>[2x]GSWEIDPKDLTFLKELGTGQFGVVKYGKWRGQYDVAIKMIKEGSMSEDEFIEEAKVMMNLSHEKLVQLYGVCTKQRPIFIITEYMANGCLLNYLREMRHRFQTQQLLEMCKDVCEAMEYLESKQFLHRDLAARNCLVNDQGVVKVSDFGLSRYVLDDEYTSSVGSKFPVRWSPPEVLMYSKFS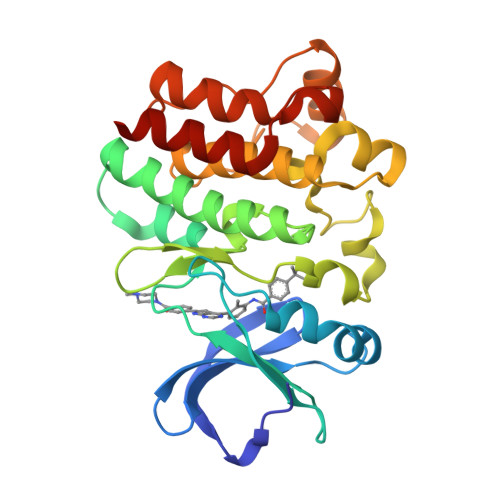SKSDIWAFGVLMWEIYSLGKMPYERFTNSETAEHIAQGLRLYRPHLASEKVYTIMYSCWHEKADERPTFKILLSNILDVMDEE> GSTAPPTNQWYHGKLDRTIAEERLRQAGKSGSYLIRESDRRPGSFVLSFLSQMNVVNHFRIIAMSGDYYIGGRRFSSLSDLIGYYSHVSSLLKGEKLLYPVAPPEPVEDRRRVRAILPYTKVPDTDEISFLKGDMFIVHNELEDGWMWVTNLRTDEQGLIVEDLVEEVGREEDPHEGKIWFHGKISKQEAYNLLMTVGQVSSFLVRPSDNTPGDYSLYFRTNENIQRFKISPTPNNQFMMGGR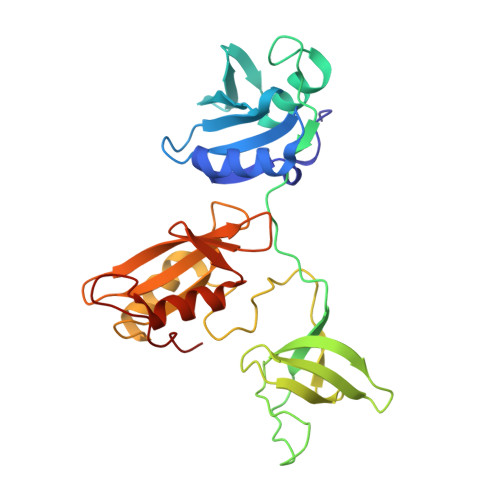YYNSIGDIIDHYRKEQIVEGYYLKEPVPMQ> STKFSDNYDVKEELGKGAFSVVRRCVHKTTGLEFAAKIINTKKLSARDFQKLEREARICRKLQHPNIVRLHDSIQEESFHYLVFDLVTGGELFEDIVAREFYSEADASHCIQQILESIAYCHSNGIVHRNLKPENLLLASKAKGAAVKLADFGLAIEVNDSEAWHGFAGTPGYLSPEVLKKDPYSKPVDIWACGVILYILLVGYPPFWDEDQHRLYAQIKAGAY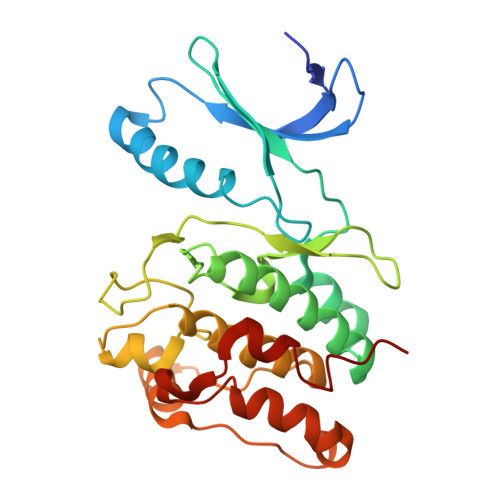DYPSPEWDTVTPEAKSLIDSMLTVNPKKRITADQALKVPWICNRE>[2x]MVELTEIKDDVVQLDEPQFSRNQAIVEEKASATNNDVVDDEDDSDSDFEDEFDENETLLDRIVALKDIVPPGKRQTISNFFGFTSSFVRNAFTKSGNLAWTLTTTALLLGVPLSLSILAEQQLIEMEKTFDLQSD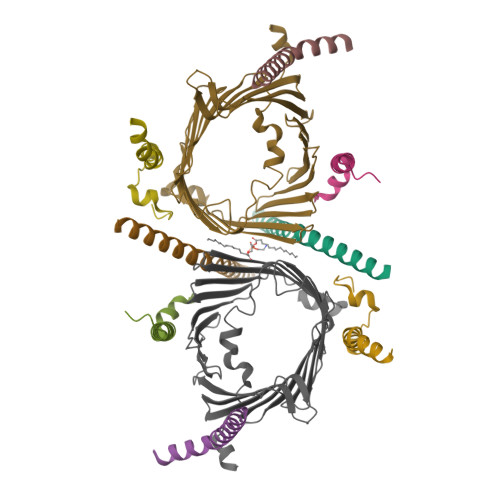ANNILAQGEKDAAATAN;>MFGLPQQEVSEEEKRAHQEQTEKTLKQAAYVAAFLWVSPMIWHLVKKQWK[2x];>MDGMFAMPGAAAGAASPQQPKSRFQAFKESPLYTIALNGAFFVAGVAFIQSPLMDMLAPQL[2x];>[2x]MSFLPSFILSDESKERISKILTLTHNVAHYGWIPFVLYLGWAHTSNRPNFLNLLSPLPSV;>MSAPTPLAEASQIPTIPALSPLTAKQSKGNFFSSNPISSFVVDTYKQLHSHRQSLELVNPGTVENLNKEVSRDVFLSQYFFTGLRADLNKAFSMNPAFQTSHTFSIGSQALPKYAFSALFANDNLFAQGNIDNDLSVSGRLNYGWDKKNISKVNLQISDGQPTMCQLEQDYQASDFSVNVKTLNPSFSEKGEFTGVAVASFLQSVTPQLALGLETLYSRTDGSAPGDAGVSYLTRYVSKKQDWIFSGQLQANGALIASLWRKVAQNVEAGIETTLQAGMVPITDPLMGTPIGIQPTVEGSTTIGAKYEYRQSVYRGTLDSNGKVACFLERKVLPTLSVLFCGEIDHFKNDTKIGCGLQFETAGNQELLMLQQGLDADGNPLQALPQL[2x]> MSYQVLARKWRPQTFADVVGQEHVLTALANGLSLGRIHHAYLFSGTRGVGKTSIARLLAKGLNCETGITATPCGVCDNCREIEQGRFVDLIEIDAASRTKVEDTRDLLDNVQYAPARGRFKVYLIDEVHMLSRHSFNALLKTLEEPPEHVKFLLATTDPQKLPVTILSRCLQFHLKALDVEQIRHQLEHILNEEHIAHEPRALQLLARAAEGSLRDALSLTDQAIASGDGQVSTQAVSAMLGTLDDDQALSLVEAMVEANGERVMALINEAAARGIEWEALLVEMLGLLHRIAMVQLSPAALGNDMAAIELRMRELARTIPPTDIQLYYQTLLIGRKELPYAPDRRMGVEMTLLRALA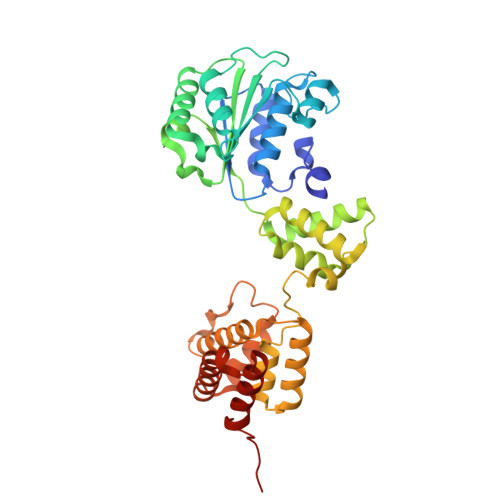FHPRMPLPEP> NTGCYGIP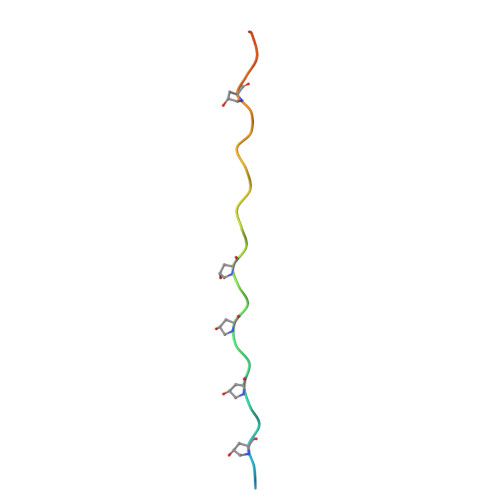GMPGLPGAPGKDGYDGLPGPKGEPGIP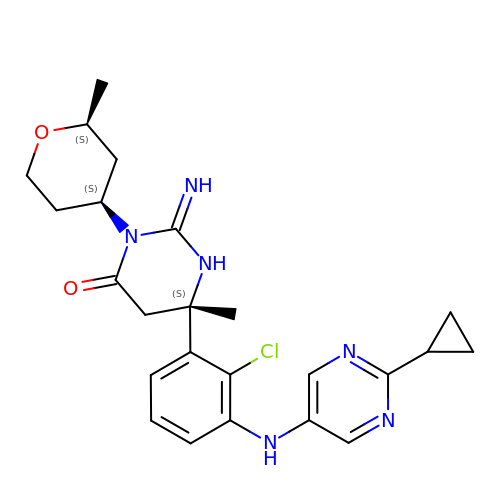(2E,6S)-6-{2-chloro-3-[(2-cyclopropylpyrimidin-5-yl)amino]phenyl}-2-imino-6-methyl-3-[(2S,4S)-2-methyloxan-4-yl]-1,3-diazinan-4-one | C24 H29 Cl N6 O2 | RUZADINCVKIRSK-NPALWHDTSA-N ACETOACETYL-COENZYME A | C25 H40 N7 O18 P3 S | 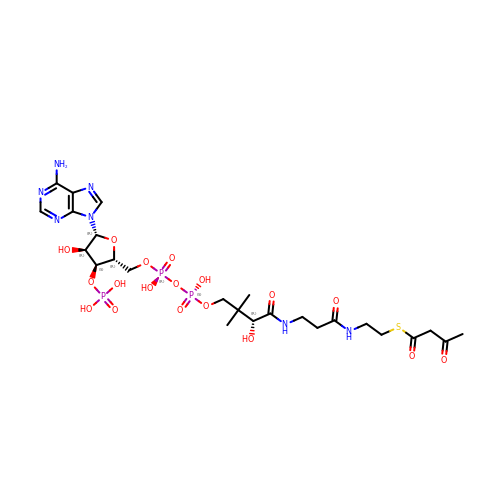OJFDKHTZOUZBOS-CITAKDKDSA-N>GAMNNTIINSLIGGDDSIKRSNVFAVDSQIPTLYMPQYISLSGVMTNDGPDNQAIASFEIRDQYITALNHLVLSLELPEVKGMGRFGYVPYVGYKCINHVSISSCNGVIWEIEGEELYNNCINNTIALKHSGYSSELNDISIGLTPNDTIKEPSTVYVYIKTPFDVEDTFSSLKLSDSKITVTVTFNPVSDIVIRDSSFDFETFNKEFVYVPELSFIGYMVKNVQIKPSFIEKPRRVIGQINQPTATVTEVHAATSLSVYTKPYYGNTDNKFISYPGYSQDEKDYIDAYVSRLLDDLVIVSDGPPTGYPESAEIVEVPEDGIVSIQDADVYVKIDNVPDNMSVYLHTNLLMFGTRKNSFIYNISKKFSAITGTYSDATKRTIFAHISHSINIIDTSIPVSLWTSQRNVYNGDNRSAESKAKDLFINDPFIKGIDFKNKTDIISRLEVRFGNDVLYSENGPISRIYNELLTKSNNGTRTLTFNFTPKIAFRPTTITANVSRGKDKLSVRVVYSTMDVNHPIYYVQKQLVVVCNDLYKVSYDQGVSITKIMGDNN[3x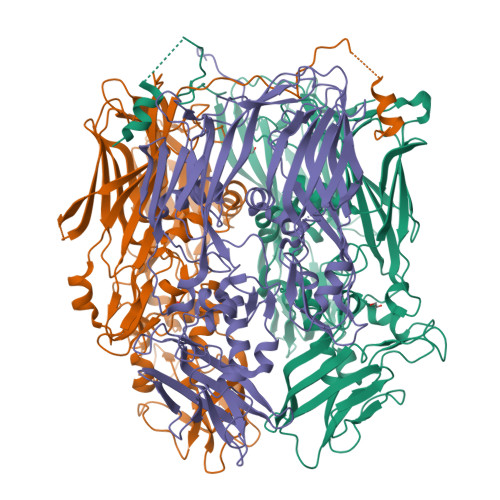]> GITTPEEMIEKAKGETAYLPCKFTLSPEDQGPLDIEWLISPADNQKVDQVIILYSGDKIYDDYYPDLKGRVHFTSNDLKSGDASINVTNLQLSDIGTY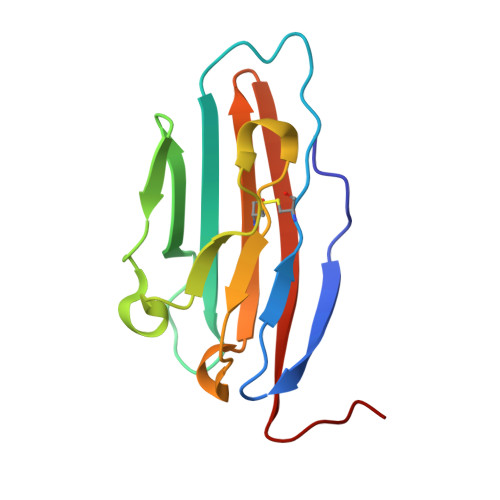QCKVKKAPGVANKKIHLVVLVKPSGA> MKDSGDSKDQQLMVALRVRPISVAELEEGATLIAHKMDEQMVVLMDPMEDPDDILRAHRSREKSYLFDVAFDFTATQEMVYQATTKSLIEGVISGYNATVFAYGPTGCGKTYTMLGTDHEPGIYVRTLNDLFRAIEETSNDMEYEVSMSYLEIYNEMIRDLLNPALGYLELREDSKGVIQVAGITEVSTINAKEIMQLLMKGNRQRTQEPTAANQTSSRSHAVLQVAVRQRSRVKNILQEVRQGRLFMIDLAGSERASQTQNRGQRMKEGAHINRSLLALGNCINALSDKGSNKYINYRDSKLTRLLKDSLGGNSRTVMIAHISPASTAFEESR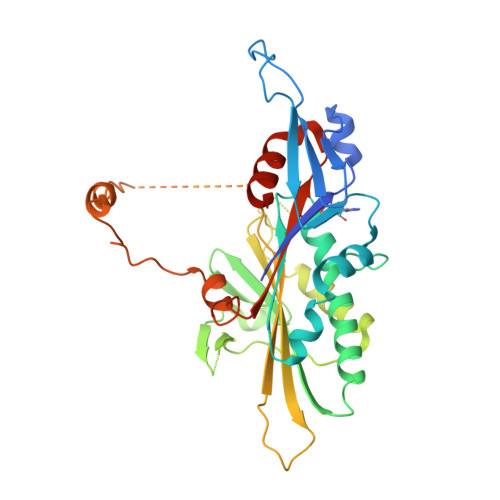NTLTYAGRAKNIRTRVKQN(9cis)-retinoic acid | 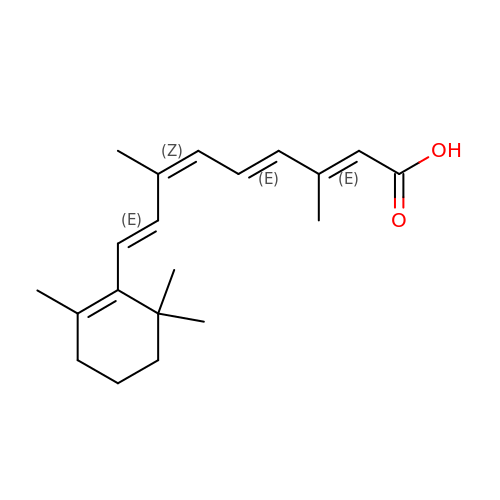C20 H28 O2 | SHGAZHPCJJPHSC-ZVCIMWCZSA-N TRPM2 belongs to the M (Melastatin) subfamily of transient receptor potential (TRP) ion channels. TRPM2 is a Ca2+ permeable non-selective cation channel opened by simultaneous binding of three obligate co-activators, cytosolic ADP-ribose (ADPR), Ca2+, and membrane phosphatidylinositol 4,5-bisphosphate (PIP2). Similarly to other TRPM subfamily channels, homotetrameric TRPM2 channels contain an ~800 residue N-terminal region, a transmembrane domain (TMD), a TRP domain, and a coiled-coil. In TRPM2 a C-terminal ~270 residue NUDT9-homology (NUDT9H) domain serves to bind ADPR.

Here, we determined the structure of the TRPM2 channel from the cnidarian Nematostella vectensis (nvTRPM2) in complex with Ca2+ by electron cryo-microscopy (cryo-EM), at a resolution of 3.1 Å, and correlated the structure with detailed biophysical characterization of channel permeation and gating properties. The C-terminal NUDT9H domain, however, is entirely invisible in the density map, indicating that in the absence of ADPR this domain is flexibly linked to the core structure. The selectivity filter is short and wide, the diameter at its narrowest point is ~5.2 Å, larger than that of TRPM4 (~4.2 Å). The nvTRPM2 filter is lined by the backbone atoms of Y1035 and G1036, and the side chain of E1037. The external vestibule of nvTRPM2 is lined by a double ring of negative charges, the side chains of D1041 and E1042 of the post-filter helix (LDE motif, inset), and additional negatively charged side chains (E1046 and E1050) line the upper parts of the vestibule. As observed in other TRPM family channels, the gate of nvTRPM2 is formed by the S6 bundle crossing which constricts the pore to a diameter of less than 2 Å between residues I1082 and N1086. Because that diameter is too small to allow passage of a water molecule, the observed nvTRPM2 conformation must correspond to a closed gate, as expected in the absence of ADPR. Although the nvTRPM2 structure was obtained in the presence of trace amounts of Ca2+ (free Ca2+ concentration in an unbuffered saline with no added Ca2+ is in the micromolar range, for example, [Csanády and Adam-Vizi, 2003]), clear density for a bound Ca2+ ion is seen, occluded into each subunit. The Ca2+ binding site, formed by the cytosolic ends of transmembrane helices S2 and S3, and the S2-S3 linker helix, is located at the membrane-cytosol interface, and is accessible from the protein surface through a narrow opening (‘peripheral tunnel’). The bound Ca2+ ion is coordinated by the side chains of residues E893 and Q896 of S2 and N918 and D921 of S3 in a pentacovalent geometry, E893 provides two coordinate bonds to the ion.

>MGKDSFTPLYDGGDSSHVHLNKFGSNQLSQSKKSWIARNFSRRECIRFVPKSHDVSRCKCGRPRERHSQQALESGQGSEEWNVASCTTKHPTNAYGEIDFEGYGGQKRAPYLRMSHDTDANLVITLMLKRWNLEIPNLVISVTGGAKSFVLKPRLREMFRRGLIKAAKTTGAWIITGGTNTGVMKHVGEAVKEQQLMFGSDTQVNVIGIATWGIVDKQSDLISEKNGKYPALYSMEPTPGHQGAMLDPNHSHFFLVDDGTEGKYGVEIGMRSRIEEAIMKVKTDSRSEAGSIGVPVVLLVLEGGPNTVATMYELIKKKVPAVVIDGSGRAASVVGFAYNHTIKRNVDGQTINVIDPQYEDEVRAKVVEVFGAKGADKTYSMIKDVLEDEKMISVYSLDGEISQDIDLAILKALLKANRSSPVAQLNLALAWNRIDLAKSDIFTEEQQWTTETLSAAMLTALLDDKAEFAELFLQNGLSMREFLSLDILCKLYAEVPGNTTIKPLLQKEMGKRQVKTIDMDVVGEVIEELMGDMFESYYRKDGHYFGELASYAEGLVLKNRKSSKDLLANINRIDPLPTPYLDVFLWAVLCNRRELARVLWEAGREPMAAALMASRLLKRMASRAQEDNTITDISSDLYDHARLFEERAVGVLDECFNENETLSQTLLVRELDHYSRMTALELAVSAESQDFIAHTSCQVLLTRLWMGTMAMNTRWWKVLVCLYLPVLIFPIIYFVPDEQHERQAAEREHQKSLNQKSSKVKSHKEKNDAPVVPVYRSKEEKAVSNDEEARVGTENEEEDFQLEDYIPEIREDDSMEVIMRNKKLGFCDRIMHFYSAPFSKFVGNVVGYLAFIFLYAYVVLFNFPRFDPAKTLGGIHPTEIVLYFWVFTILIEEIRQLAAKPPKYIKDKVSVYFSDTWNFVDIFSLTVFIIAIILRFFTNSRIFTASRIILSLDIIFFIVRSLQIFSVNRLLGPKLVMIQKMMQDLAQFIIILAVFTIAYGIALHAVMFPSPGIYARNNTWVTITSVVQYPYWQMYGELFLDEIQGEKPKEFGEVDPDGRWLSPLLLAIYMVFTNILLLNLLIAIFNYTFERVQEDSDKVWKFQRYDLVQEYHSRPVFAPPLVLLGHILIFIRWVWRMCRCGHPPRGSTMKIGLSPAEMEQMDNWEFQAAEMYIHQQQQKNSGTLEERVRALGDRVDCINSQLNRVLDSMSGTRAHALTDGNGLEGGHDSEGRLARMEVELSSNSESLQKILALLQQQPPVKGQAAVPIQLTLLHYKARSSPYPGSTAKRFAVQDNMVDWQVPFPDYKPVNYTAPVVLANPVWADKDLMAMSPRPELPYNQMDHTCNVNRVSYNGTYVVKDGLPLNPMGRTGMQGRGLLGRFGPNHAADPVVTRWKRTSAGVMLQGGKKVLEFVAIQRKDNNQWAIPGGMVEPGQLVTQALKAEFGEEAMAKLNVSQEEKERIAKQIERLFQQGQEIYKGYVDDPRNTDNAWMETVAVNFHDDKGDLFGDITLQAGDDAAAVRWQRVSGNIPLYASHVSILEKVAKMRDAAFSNSLEVLFQ[4x]> YDGTHC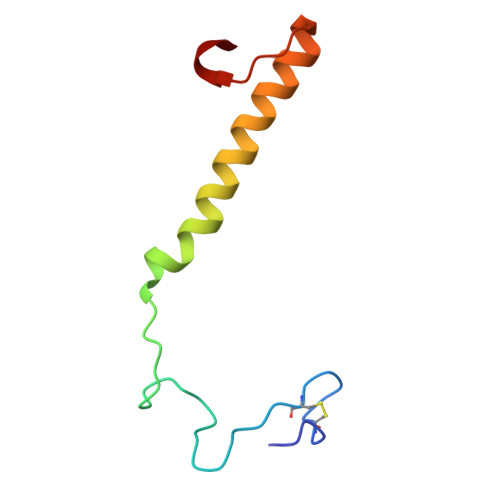KAPGNCWEPKPGYPDKVAGSKYDPKHDPNELNKQAESIKAMEARNQKRVENYAKTGKFVYKVEDIK S-BENZYL-GLUTATHIONE 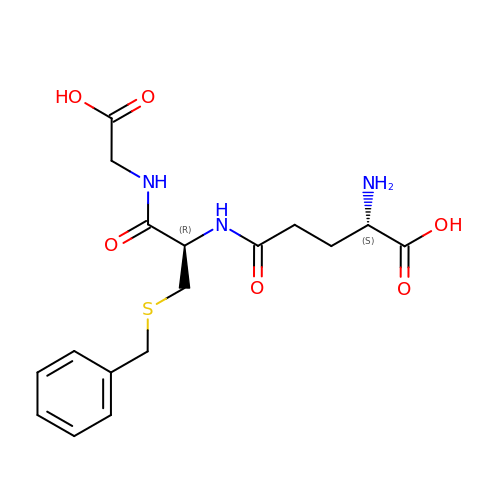| C17 H23 N3 O6 S | XYJWEQWNNKNSFU-STQMWFEESA-N>[3x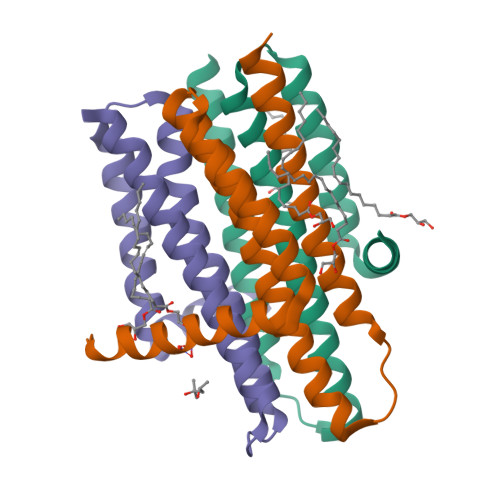]GHHHHHHELANNTTGFTRIIKAAGYSWKGLRAAWINEAAFRQEGVAVLLAVVIACWLDVDACTRVLLISSVMLVMIVELLNSAIEAVVDRIGSEYHELSGRAKDLGSAAVLIAIIDAVITWCILLWSHFG> GSHMKVEDPKDFPSELLSFLSHAVFSNRTLACFAIYTTKEKAALLYKKIMEKYSVTFISR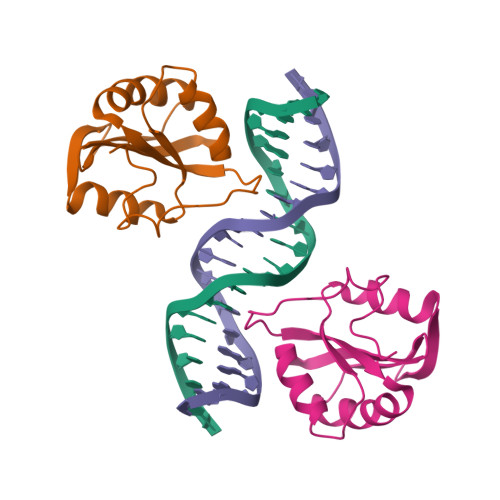HNSYNHNILFFLTPHRHRVSAINNYAQKLSTFSFLICKGVNKEYLMYSALTRDPFSVIEESLPGGLKEHDFNP ETHYL (4R)-4-({N-[(BENZYLOXY)CARBONYL]-L-PHENYLALANYL}AMINO)-5-[(3S)-2-OXOPYRROLIDIN-3-YL]PENTANOATE 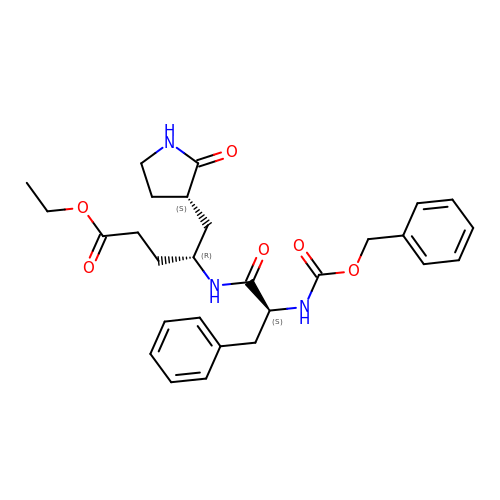| C28 H35 N3 O6 | PIZHLOUXQJUQHF-VXNXHJTFSA-N>MGSDKIHHHHHHENLYFQGMNFQMNEAIQLLE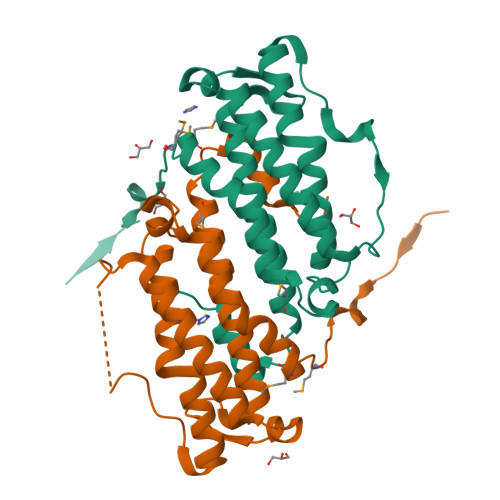RTPKTLEVFLEGLSDSWHQCNEGYETWTVYEVVVHLIEAEKTNWIPRLRFILQEGEHKPFPAFDRFSHLNQSNAVPISERFKEFQQLRKENLNTLRSLVQSEADLERTGAHPAFGVVKVRELLSAWVVHDLTHIAQIVRSMAKRYDTDVGPWKEYLGILND[4x]> ADLSELLKEGTKEAHDRAENTQFVKDFLKGNIKKELFKLATT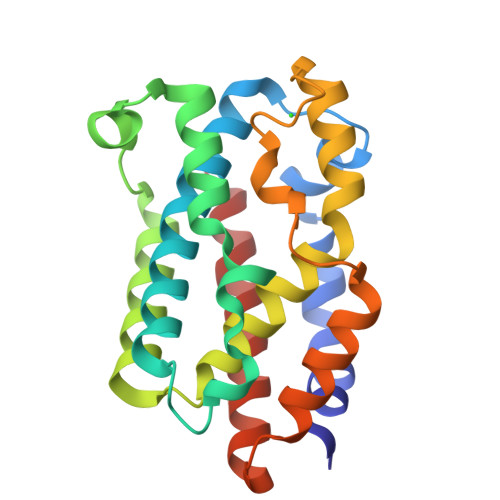ALYFTYSALEEEMERNKDHPAFAPLYFPMELHRKEALTKDMEYFFGENWEEQVQCPKAAQKYVERIHYIGQNEPELLVAHAYTRYMGDLSGGQVLKKVAQRALKLPSTGEGTQFYLFENVDNAQQFKQLYRARMNALDLNMKTKERIVEEANKAFEYNMQIFNEL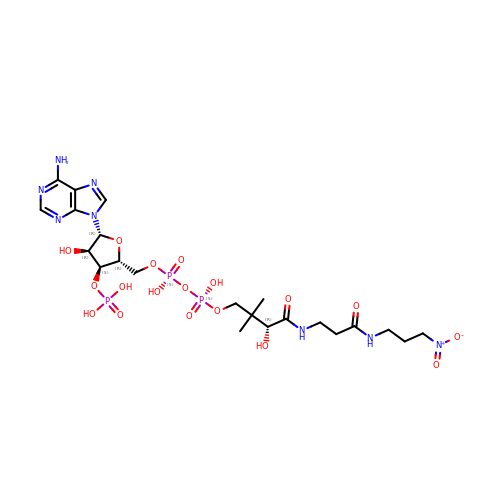NITROMETHYLDETHIA COENZYME A | C22 H37 N8 O18 P3 | PUGKTLRHGHIDCJ-GORZOVPNSA-N In bacteria and archaea, chromosome dimers are monomerized by members of a large family of tyrosine recombinases, the Xer recombinases. Many other organisms (including Lactococcus, Helicobacter, Campylobacter spp. and archaea) employ a single Xer recombinase system, with a prime example, XerH/difH, found in Helicobacter pylori, a gastric pathogen implicated in peptic ulcer disease and gastric cancer. Xer recombinases are members of the tyrosine site-specific recombinase superfamily, a large group of enzymes that catalyze DNA breakage and rejoining using a conserved tyrosine nucleophile. Here, we present two crystal structures of the H. pylori XerH recombinase in complex with its recombination site difH.

We then co-crystallized full-length wild-type XerH with a 30 bp difH DNA duplex. The resulting 2.1 Å resolution structure shows a synaptic complex with two difH molecules and four XerH subunits. Each difH site interacts with two XerH molecules, one molecule (molecule A) binding to the left arm and one (molecule B) to the right arm. The two domains of each subunit form a tight, C-shaped clamp around one arm of the difH site. Perhaps the most unexpected feature of the XerH-difH synaptic complex structure is the DNA conformation, which is nearly straight. Both DNA molecules in the synapse resemble B-form DNA, with a wide angle (165°) between the two difH arms. Instead, the main difference in the recognition of the two arms involves a conserved thymine base (T4/T5') in the outer parts of the arms: In the left arm, T4 forms hydrophobic contacts with XerH αK and makes a specific hydrogen bond with lysine K290 (red insert), whereas in the right arm T5' is closer to the center of difH and cannot make these interactions. While the αN-αO segment of molecule A is fully ordered, the linker and αO are partially disordered in molecule B. Also, helices αO point in different directions (~100° rotation). The catalytic tyrosine Y344 is far away (5.2–5.8 Å) from the scissile phosphate in all subunits, so the structure represents a catalytically inactive synaptic complex, implying a conformational change is required prior to catalysis. The pre-cleavage synaptic complex crystal structure contains nearly straight difH DNA, and XerH is in a catalytically inactive conformation.

>SMKHPLEELKDPTENLLLWIGRFLRYKCTSLSNSQVKDQNKVFECLNELNQACSSSQLEKVCKKARNAGLLGINTYALPLLKFHEYFSKARLITERLAFNSLKNIDEVMLAEFLSVYTGGLSLATKKNYRIALLGLFSYIDKQNQDENEKSYIYNITLKNISGVNQSAGNKLPTHLNNEELEKFLESIDKIEMSAKVRARNRLLIKIIVFTGMRSNEALQLKIKDFTLENGCYTILIKGKGDKYRAVMLKAFHIESLLKEWLIERELYPVKNDLLFCNQKGSALTQAYLYKQVERIINFAGLRREKNGAHMLRHSFATLLYQKRHDLILVQEALGHASLNTSRIYTHFDKQRLEEAASIWEEN[4x]> MFAKLHGKKQRPISSINSQTPRTSNTTHANSISLSSGNLIVGSNRNLRQKKEQFGSQQRASGRKLISNKENDDNVNNGGDNNYDNGERVHRHHIPGLKIKAYQAELGYHESRFSENLVMLNLVEFPDIKPGDLVELKTYHKNPSASNGDKKIYFIAKDFDGETKRRAKTSNVSILSGQLQTLLDLPSRSRIWIKLKPNKFDLQADVVEFNIKDCLLNRGDMWVLSSKLVDTCVFMDQRLAFLDSIRGTIKGIYRNGKKIVSGYIGEQTRIIFRSESARLIFLIQITDEMWNFEETGEQLFQKMVNSFFPKIFKKWKDVDTHHTITIAFAISMDLSDTSFKDLTPGESLKNSQDYFRIVVDQVSIIHWVDIMETLREEFMEIRKDLLNKQTDKGYSVANGRFSPVIKSNFLELVNFATTILTDPFKQLDLRHTTTHVMIISPGSGLFDVDYSLLRLTGKKLLSLEMTMDLICLSKAPLHIVPLFRYRDFENKLHHCVPLWLSVFFWNDHDKKSNSEWTPRCKIYDLQMMGITENELIREVDVEYLQLNKKVKSLSEFMNDYDKNAFEVKILCAGSNTKQSKKLNSKFDTVFENDVVVKARKIPATATTTHGNTKFIWRGPKVALPAIKDIQKPNVIPDLSIKTIEASFYDDCNTTNDKISTPTTSNNDNLEMNDSLVSVRSADNQNTSLALDSLKGLSKRNSLKDFTQRVITKFISNIDTSKNKKIKSTLLRDDVDNSPLGSNTPLPSSESKISGLKLQQKGLADENVISKRGNLIIKKNLSIFGLPSNEIMSGSPSSYLGSSHTRTSSKLSNMSDKAAFITEGQKSKHDDSNTYSLTQQLKHRISETWVDIKSPSIPVSSEFANELLPIRWKDVWPKYVARKYSKWRSFTTPAELPITISDFPSKDDFDRNFIFRNHSVTLNTDQEQYNQTYKDLLRDMIYMRLLTGFQICVGRQVEKIELSRESGESETVVNKYLDFNQNDAFKLYLMIDSEIHRITCSSSGIIDVERYLRKDEANLFDQVPSYIPLVKTRYESSFRDAMIDPLHVKRESLNWNQIDQVLAGYGDNLIDRKWHGFRAKYVVLPTDIPPNTYSMVINGKSETLNPEEIRVEGLRRLIGSITRSRLRTEKEKKGRKTKREEIQPEVMFYTGPLYNFINEQQTSLESSAINFKDSIFVNDNNLLNRNVELSKLAYQIQRGEDRITLVNRKWHWKKHEKCFVGSEMVNWLIRNFSDIDTREDAIKYGQKVMKEGLFVHVLNKHNFLDGHYFYQFSPEYVMDTNKLEKTNSHRSTLSDPKQMLRKASTGSSNDPSAMTPFSSVVPAISASNASVADAKEPSRPILMLSNSLVIDVDPAGKSSKQESCTVHYDRVHNPDHCFHIRLEWLTTTPKLIDDLVGNWSRLCERYGLKMIEIPWEELCTIPSVNPFHSFVEIKLAINPWEDPEFKDR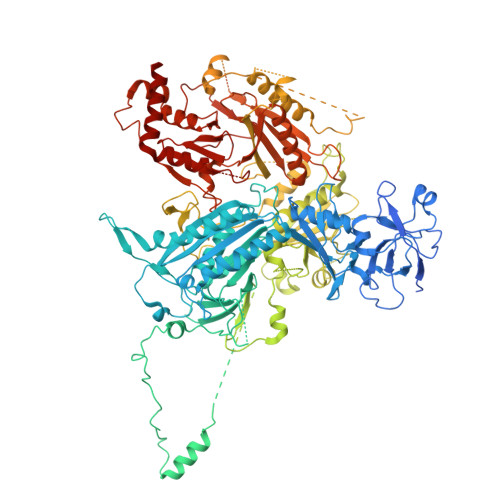ELFAKSKFYYHVYLLKASGFLLDNRASKFLQNQDIEFDIMYSWGKPQFKYVQYIHHTGAYVAELRENGCLFLAPNNIYISRVNPGNIIGKIHSASSSSLDAQKVILNFKSTCLDYQKLRSIFLDAKEMWITGKIVED The biosynthesis of the lincosamide antibiotics lincomycin A and celesticetin involves the pyridoxal-5′-phosphate (PLP)-dependent enzymes LmbF and CcbF, which are responsible for bifurcation of the biosynthetic pathways. Despite recognizing the same S-glycosyl-l-cysteine structure of the substrates, LmbF catalyses thiol formation through β-elimination, whereas CcbF produces S-acetaldehyde through decarboxylation-coupled oxidative deamination. To understand the molecular basis for the differences between LmbF and CcbF, we solved the X-ray crystal structures of LmbF and CcbF with PLP at resolutions of 1.7 Å and 1.8 Å, respectively. In the active sites of LmbF and CcbF, the PLP is covalently bound to the catalytic Lys270 and Lys260 residues, respectively, to form internal aldimines.

In the LmbF active site, the N1 and C3-hydroxy groups of PLP interact with Asp233 and Asn205, respectively, and the phosphate group of PLP hydrogen-bonds with Thr122, Ser267 and Ser269. Moreover, Trp150 interacts with the pyridine ring of PLP by π–π interactions. Although the residues lining the active-site cavity are in comparable positions, Asn205, Phe236, Leu83′ and Pro302′ in LmbF are uniquely substituted with Tyr195, Tyr226, Tyr72′ and Tyr292′ in CcbF, respectively. Docking of the external aldimine intermediate of 4 into the active site of LmbF and 50-ns simulations showed hydrogen-bond interactions involving the carboxylate group of the cysteine moiety of 4, the C3-hydroxy group of PLP, and Asn205. The dihedral ϕ angle between the Cα–H bond and pyridine ring of PLP is stably maintained around −70° to −90°, indicating that the Cα–H bond is aligned parallel to the p orbitals of the conjugated π-system. The dihedral angle of N–Cα–C–S is −65°, and the octose moiety of 4 is within a pocket consisting of Leu83′, Pro302′, Thr303′ and PLP. As a result, the ε-amino group of Lys270 remains within ~2.5–3.5 Å of the Cα H atom, and the distance between the ε-amino group of Lys270 and the S atom of 4 is less than 3.5 Å in the calculation, suggesting that Lys270 probably acts as an acid–base catalyst to facilitate the C–S bond cleavage. The in vitro enzyme reactions of the LmbF L83Y, W150A, N205Y, F236Y, K270A and P302Y variants revealed that the β-elimination activity is abolished or dramatically decreased in most cases (less than 10% compared to wild type), except for the L83Y and F236Y variants, which showed 21% and 58% activities, respectively. Although most of the multiple-site mutations at Leu83′, Asn205, Phe236 and Pro302′ of LmbF merely reduced or abolished the β-elimination activity, the LmbF L83Y/F236Y variant catalysed the decarboxylation-coupled oxidative amidation to produce 9, as well as the β-elimination reaction. Leu83′ and Phe236 in LmbF influence the selectivity between β-elimination and oxidative amidation.

>[2x]MTATASGAQTAAPERLTDDGWLIRRTSVDTVRPFDDPSAQWMLDRAQARLPLYLLHVADHAEATPPGLREALHAQDAAPCDGLLFSQYGLPELRRRLDAWLAADEEWDTAAEPLVSVAWSGTGAAIFDLLRMLKDGRPGPSAVLLPRPGWGYDMSVRDTGHVPVSYEVPPESPHGPDPAHLEEAWQRCRSEGLDVACILINPQHNPWGGNWTPEFLAAVAALAERERVPVLVDNAFYGLTAEDVRPTSAVRLLGHLVGQELLVSVRSLSKQFACSGWALGAVAGSPGLVSAYSGRWRCLREPTAGFRAQAAMAAWLGGAEPERFTRRRRSEATRHARLLRTTLRAAGLPDDAVLHHGGAPFTLLRPPGGSTVEEVREQTVVRHGVLLGLERDARERPWFKVWLGRDSSVFEPAARALGDAAAEWRYRLEHHHHHHHH> MKPEVEQELAHILLTELLAYQFASPVRWIETQDVFLKDFNTERVVEIGPSPTLAGMAQRTLKNKYESYDAALSLHREILCYSKDAKEIYYTPDPSELAAKEEPAKEEAPAPTPAASAPAPAAAAPAPVAAAAPAAAAAEIADEPVKASLLLHVLVAHKLKKSLDSIPMSKTIKDLVGGKSTVQNEILGDLGKEFGTTPEKPEETPLEELAETFQDTFSGALGKQSSSLLSRLISSKMPGGFTITVARKYLQTRWGLPSGRQDGVLLVALSNEPAARLGSEADAKAFLDSMAQKYASIVGVDLSSAASASGAAGAGAAAGAAMIDAGALEEITKDHKVLARQQLQVLARYLKMDLDNGERKFLKEKDTVAELQAQLDYLNAELGEFFVNGVATSFSRKKARTFDSSWNWAKQSLLSLYFEIIHGVLKNVDREVVSEAINIMNRSNDALIKFMEYHISNTDETKGENYQLVKTLGEQLIENCKQVLDVDPVYKDVAKPTGPKTAIDKNGNITYSEEPREKVRKLSQYVQEMALGGPITKESQPTIEEDLTRVYKAISAQADKQDISSSTRVEFEKLYSDLMKFLESSKEIDPSQTTQLAGMDVEDALDKDSTKEVASLPNKSTISKTVSSTIPRETIPFLHLRKKTPAGDWKYDRQLSSLFLDGLEKAAFNGVTFKDKYVLITGAGKGSIGAEVLQGLLQGGAKVVVTTSRFSKQVTDYYQSIYAKYGAKGSTLIVVPFNQGSKQDVEALIEFIYDTEKNGGLGWDLDAIIPFAAIPEQGIELEHIDSKSEFAHRIMLTNILRMMGCVKKQKSARGIETRPAQVILPMSPNHGTFGGDGMYSESKLSLETLFNRWHSESWANQLTVCGAIIGWTRGTGLMSANNIIAEGIEKMGVRTFSQKEMAFNLLGLLTPEVVELCQKSPVMADLNGGLQFVPELKEFTAKLRKELVETSEVRKAVSIETALEHKVVNGNSADAAYAQVEIQPRANIQLDFPELKPYKQVKQIAPAELEGLLDLERVIVVTGFAEVGPWGSARTRWEMEAFGEFSLEGCVEMAWIMGFISYHNGNLKGRPYTGWVDSKTKEPVDDKDVKAKYETSILEHSGIRLIEPELFNGYNPEKKEMIQEVIVEEDLEPFEASKETAEQFKHQHGDKVDIFEIPETGEYSVKLLKGATLYIPKALRFDRLVAGQIPTGWNAKTYGISDDIISQVDPITLFVLVSVVEAFIASGITDPYEMYKYVHVSEVGNCSGSGMGGVSALRGMFKDRFKDEPVQNDILQESFINTMSAWVNMLLISSSGPIKTPVGACATSVESVDIGVETILSGKARICIVGGYDDFQEEGSFEFGNMKATSNTLEEFEHGRTPAEMSRPATTTRNGFMEAQGAGIQIIMQADLALKMGVPIYGIVAMAATATDKIGRSVPAPGKGILTTAREHHSSVKYASPNLNMKYRKRQLVTREAQIKDWVENELEALKLEAEEIPSEDQNEFLLERTREIHNEAESQLRAAQQQWGNDFYKRDPRIAPLRGALATYGLTIDDLGVASFHGTSTKANDKNESATINEMMKHLGRSEGNPVIGVFQKFLTGHPKGAAGAWMMNGALQILNSGIIPGNRNADNVDKILEQFEYVLYPSKTLKTDGVRAVSITSFGFGQKGGQAIVVHPDYLYGAITEDRYNEYVAKVSAREKSAYKFFHNGMIYNKLFVSKEHAPYTDELEEDVYLDPLARVSKDKKSGSLTFNSKNIQSKDSYINANTIETAKMIENMTKEKVSNGGVGVDVELITSINVENDTFIERNFTPQEIEYCSAQPSVQSSFAGTWSAKEAVFKSLGVKSLGGGAALKDIEIVRVNKNAPAVELHGNAKKAAEEAGVTDVKVSISHDDLQAVAVAVSTKK;> MDAYSTRPLTLSHGSLEHVLLVPTASFFIASQLQEQFNKILPEPTEGFAADDEPTTPAELVGKFLGYVSSLVEPSKVGQFDQVLNLCLTEFENCYLEGNDIHALAAKLLQENDTTLVKTKELIKNYITARIMAKRPFDKKSNSALFRAVGEGNAQLVAIFGGQGNTDDYFEELRDLYQTYHVLVGDLIKFSAETLSELIRTTLDAEKVFTQGLNILEWLENPSNTPDKDYLLSIPISCPLIGVIQLAHYVVTAKLLGFTPGELRSYLKGATGHSQGLVTAVAIAETDSWESFFVSVRKAITVLFFIGVRCYEAYPNTSLPPSILEDSLENNEGVPSPMLSISNLTQEQVQDYVNKTNSHLPAGKQVEISLVNGAKNLVVSGPPQSLYGLNLTLRKAKAPSGLDQSRIPFSERKLKFSNRFLPVASPFHSHLLVPASDLINKDLVKNNVSFNAKDIQIPVYDTFDGSDLRVLSGSISERIVDCIIRLPVKWETTTQFKATHILDFGPGGASGLGVLTHRNKDGTGVRVIVAGTLDINPDDDYGFKQEIFDVTSNGLKKNPNWLEEYHPKLIKNKSGKIFVETKFSKLIGRPPLLVPGMTPCTVSPDFVAATTNAGYTIELAGGGYFSAAGMTAAIDSVVSQIEKGSTFGINLIYVNPFMLQWGIPLIKELRSKGYPIQFLTIGAGVPSLEVASEYIETLGLKYLGLKPGSIDAISQVINIAKAHPNFPIALQWTGGRGGGHHSFEDAHTPMLQMYSKIRRHPNIMLIFGSGFGSADDTYPYLTGEWSTKFDYPPMPFDGFLFGSRVMIAKEVKTSPDAKKCIAACTG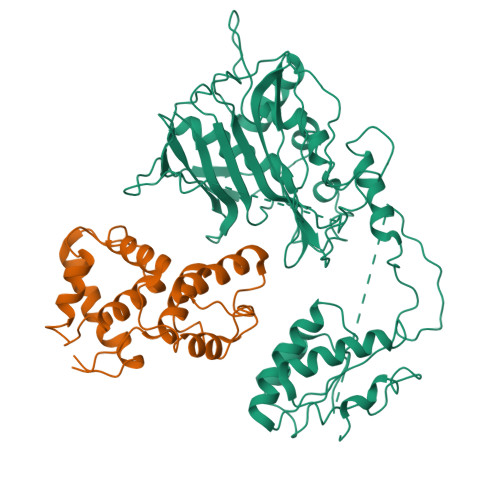VPDDKWEQTYKKPTGGIVTVRSEMGEPIHKIATRGVMLWKEFDETIFNLPKNKLVPTLEAKRDYIISRLNADFQKPWFATVNGQARDLATMTYEEVAKRLVELMFIRSTNSWFDVTWRTFTGDFLRRVEERFTKSKTLSLIQSYSLLDKPDEAIEKVFNAYPAAREQFLNAQDIDHFLSMCQNPMQKPVPFVPVLDRRFEIFFKKDSLWQSEHLEAVVDQDVQRTCILHGPVAAQFTKVIDEPIKSIMDGIHDGHIKKLLHQYYGDDESKIPAVEYFGGESPVDVQSQVDSSSVSEDSAVFKATSSTDEESWFKALAGSEINWRHASFLCSFITQDKMFVSNPIRKVFKPSQGMVVEISNGNTSSKTVVTLSEPVQGELKPTVILKLLKENIIQMEMIENRTMDGKPVSLPLLYNFNPDNGFAPISEVMEDRNQRIKEMYWKLWIDEPFNLDFDPRDVIKGKDFEITAKEVYDFTHAVGNNCEDFVSRPDRTMLAPMDFAIVVGWRAIIKAIFPNTVDGDLLKLVHLSNGYKMIPGAKPLQVGDVVSTTAVIESVVNQPTGKIVDVVGTLSRNGKPVMEVTSSFFYRGNYTDFENTFQKTVEPVYQMHIKTSKDIAVLRSKEWFQLDDEDFDLLNKTLTFETETEVTFKNANIFSSVKCFGPIKVELPTKETVEIGIVDYEAGASHGNPVVDFLKRNGSTLEQKVNLENPIPIAVLDSYTPSTNEPYARVSGDLNPIHVSRHFASYANLPGTITHGMFSSASVRALIENWAADSVSSRVRGYTCQFVDMVLPNTALKTSIQHVGMINGRKLIKFETRNEDDVVVLTGEAEIEQPVTTFVFTGQGSQEQGMGMDLYKTSKAAQDVWNRADNHFKDTYGFSILDIVINNPVNLTIHFGGEKGKRIRENYSAMIFETIVDGKLKTEKIFKEINEHSTSYTFRSEKGLLSATQFTQPALTLMEKAAFEDLKSKGLIPADATFAGHSLGEYAALASLADVMSIESLVEVVFYRGMTMQVAVPRDELGRSNYGMIAINPGRVAASFSQEALQYVVERVGKRTGWLVEIVNYNVENQQYVAAGDLRALDTVTNVLNFIKLQKIDIIELQKSLSLEEVEGHLFEIIDEASKKSAVKPRPLKLERGFACIPLVGISVPFHSTYLMNGVKPFKSFLKKNIIKENVKVARLAGKYIPNLTAKPFQVTKEYFQDVYDLTGSEPIKEIIDNWEKYEQSHHHHHH> MHHHHHHSSGRENLYFQGTFAERYNIVCMLGKGSFGEVLKCKDRITQQEYAVKVINKASAKNKDT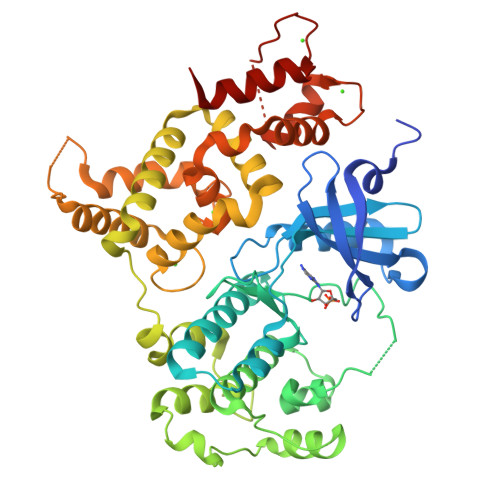STILREVELLKKLDHPNIMKLFEILEDSSSFYIVGELYTGGELFDEIIKRKRFSEHDAARIIKQVFSGITYMHKHNIVHRDLKPENILLESKEKDCDIKIIDFGLSTCFQQNTKMKDRIGTAYYIAPEVLRGTYDEKCDVWSAGVILYILLSGTPPFYGKNEYDILKRVETGKYAFDLPQWRTISDDAKDLIRKMLTFHPSLRITATQCLEHPWIQKYSSETPTISDLPSLESAMTNIRQFQAEKKLAQAALLYMASKLTTLDETKQLTEIFRKLDTNNDGMLDRDELVRGYHEFMRLKGVDSNSLIQNEGSTIEDQIDSLMPLLDMDGSGSIEYSEFIASAIDRTILLSRERMERAFKMFDKDGSGKISTKELFKLFSQADSSIQMEELESIIEQVDNNKDGEVDFNEFVEMLQNFVRNE>[16x]KSGKPSGEMDEVGVQKCKNALKLPVLEVLPGGGWDNLRNVDMGRVMELTYSNCRTTEDGQYIIPDEIFTIPQKQSNLEMNSEILESWANYQSSTSYSINTELSLFSKVNGKFSTEFQRMKTLQVKDQAITTRVQVRNLVYTVKINPTLELSSGFRKELLDISDRLENNQTRMATYLAELLVLNYGTHVTTSVDAGAALIQEDHLRASFLQDSQSSRSAVTASAGLAFQNTVNFKFEENYTSQNVLTKSYLSNRTNSRVQSIGGVPFYPGITLQAWQQGITNHLVAIDRSGLPLHFFINPNMLPDLPGPLVKKVSKTVETAVKRYYTFNTYPGCTDLNSPNFNFQANTDDGSCEGKMTNFSFGGVYQECTQLSGNRDVLLCQKLEQKNPLTGDFSCPSGYSPVHLLSQIHEEGYNHLECHRKCTLLVFCKTVC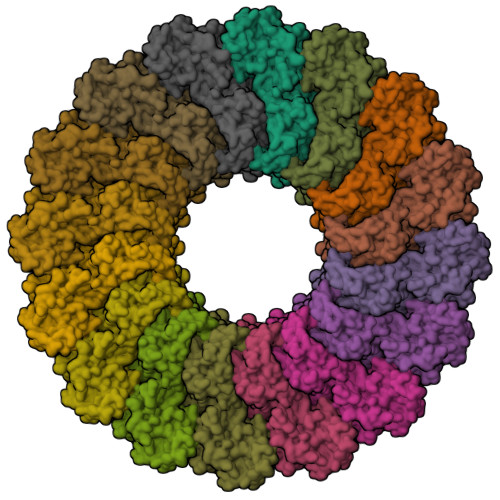EDVFQVAKAEFRAFWCVASSQVPENSGLLFGGLFSSKSINPMTNAQSCPAGYFPLRLFENLKVCVSQDYELGSRFAVPFGGFFSCTVGNPLVDPAISRDLGAPSLKKCPGGFSQHPALISDGCQVSYCVKSGLFTGGSLPPARLPPFTRPPLMSQAATNTVIVTNSENARSWIKDSQTHQWRLGEPIELRRAMNVIHGDGGGLSHHHHHH> MHHHHHHSSGLEVLFQGPGSTLVRVK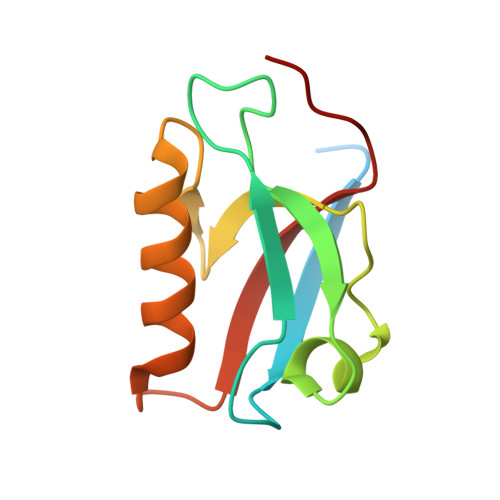KSAATLGIAIEGGANTRQPLPRIVTIQRGGSAHNCGQLKVGHVILEVNGLTLRGKEHREAARIIAEAFKTKDRDYIDFLVTEFNVML>[2x]SENDSIELDDVANLMFYGEGQIGTNKQPFMFIFDTGSANLWVPSVNCDSIGCSTKHLYDASASKSYEKDGTKVEISYGSGTVRGYFSKDVISLGDLSLPYKFIEVTDADDLEPIYSGSEFDGILGLGWKDLSIGSIDPVVVELKKQNKIDNALFTFYLPVHDKHVGYLTIGGIESDFYEGPLTYEKLNHDLYWQIDLDIHFGKYVMQKANAVVDSGTSTITAPTSFLNKFFRDMNVIK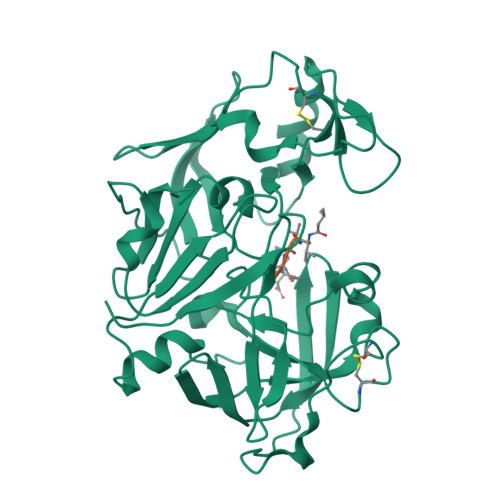VPFLPLYVTTCDNDDLPTLEFHSRNNKYTLEPEFYMDPLSDIDPALCMLYILPVDIDDNTFILGDPFMRKYFTVFDYEKESVGFAVAKNL>DVYQEPTDPKFPQQWYLSGVTQRDLNVKAAWAQGYTGHGIVVSILDDGIEKNHPDLAGNYDPGASFDVNDQDPDPQPRYTQMNDNRHGTRCAGEVAAVANNGVCGVGVAYNARIGGVRMLDGEVTDAVEARSLGLNPNHIHIYSASWGPEDDGKTVDGPARLAEEAFFRGVSQGRGGLGSIFVWASGNGGREHDSCNCDGYTNSIYTLSISSATQFGNVPWYSEACSSTLATTYSSGNQNEKQIVTTDLRQKCTESHTGTSASAPLAAGIIALTLEANKNLTWRDMQHLVVQTSKPAHLNANDWATNGVGRKVSHSYGYGLLDAGAMVALAQNWTTVAPQRKCIIDILTEPKDIGKRLEVRKTVTACLGEPNHITRLEHAQARLTLSYNRRGDLAIHLVSPMGTRSTLLAARPHDYSADGFNDWAFMTTHSWDEDPSGEWVLEIENTSEANNYGTLTKFTLVLYGTASGSLVPRGSHHHHHH[3x];>MGHHHHHHSGHMKRQFVNEWAAEIPGGPEAASAIAEELGYDLLGQIGSLENHYLFKHKNHPRKSARSAFHITKRLSDDDRVIWAEQQYEKERSKR[3x]

Proprotein convertases (PCs), including furin and PC1/3 among nine mammalian homologues, mediate the maturation of numerous secreted substrates by proteolytic cleavage. The zymogens of the furin-like PCs share a multidomain architecture comprising an N-terminal pro-domain, a subtilisin-like catalytic domain, and a P-domain (also called HomoB-domain). Activation of furin is triggered by two sequential autocatalytic cleavages and subsequent release of the prodomain. In this work, we investigate the structural and functional basis of PC-activation to engineer prodomain-based PC-inhibitors.

We created the mutant (77)R-K-S-A-R (M5) that combined these features, carrying positive charges only at positions 77,78, and 81, as well as eliminating all possible multi-basic cleavage motives (Lysine is not recognized by furin at the P4 position). In excellent agreement with the findings above, M5 (Ki = 0.042 ± 0.002 nM) was ~8-fold more potent than M2 and ~36-fold more potent than M3 as well as resistant to auto-activation. Indeed, we could obtain crystals of M5:furin and M2:furin at pH 5.9 and pH 7.0, respectively. The structures of M2:furin and M5:furin were refined to 2.0 Å and 2.4 Å resolution, respectively. Four and three copies of the PC1/3-prodomain:furin complexes were observed in the asymmetric unit for M2:furin and M5:furin, respectively. The main difference between M2:furin and M5:furin is found for the secondary cleavage site loop between Lys73 and Ala83. This region was well structured in M2:furin at pH 7.0, but no electron density was observed in M5:furin at pH 5.9. We also applied crystalline material of the M5:furin complex on a gel, showing that the prodomain was intact. Thus, protonation of His72 at pH 6.0 will change a productive interaction to an unfavored contact, probably destabilizing the conformation of the secondary cleavage site loop. Consistent with this observation, the last amino acid with visible electron density at the N-terminal end of the secondary cleavage site loop in M5:furin was His72. The structural data suggest a specific destabilization of the secondary cleavage site loop at acidic pH.>MTIDINKLKEELGLGDLAKSLEGLTAAQKAQEAERMRKEQEEKELARMNDLVSKAVGEDRKRLEEALELVKSLDEKSKKSNELFAQTVEKQQETIVGLQDEIKSLLTAREGRSFVGDSVAKALYGTQENFEDEVEKLVLLSYVMEKGVFETEHGQRHLKAVNQSSSVEVSSESYETIFSQRIIRDLQKELVVGALFEELPMSSKILTMLVEPDAGKATWVAASTYGTDTTTGEEVKGALKEIHFSTYKLAAKSFITDETEEDAIFSLLPLLRKRLIEAHAVSIEEAFMTGDGSGKPKGLLTLASEDSAKVVTEAKADGSVLVTAKTISKLRRKLGRHGLKLSKLVLIVSMDAYYDLLEDEEWQDVAQVGNDSVKLQGQVGRIYGLPVVVSEYFPAKANSAEFAVIVYKDNFVMPRQRAVTVERERQAGKQRDAYYVTQRVNLQRYFANGVVSGTYAAS[12x];>[2x]MIDYSGLRTIFGEKLPESHIFFATVAAHKYVP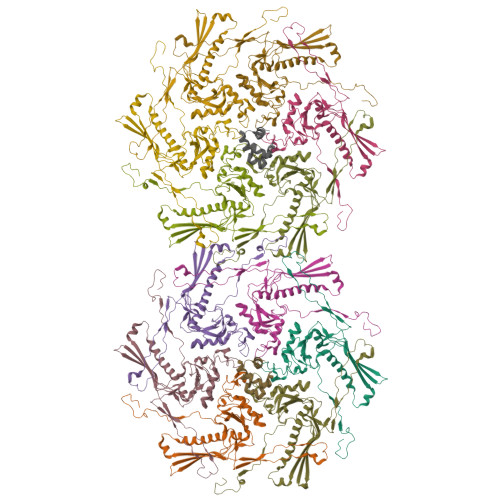SYAFLRRELGLSSAHTNRKVWKKFVEAYGKAIPPAPPAPPLTLSKDLTASMSVEEGAALTLSVTATGGTGPYTYAWTKDGSPIPDASGATYTKPTAAAEDAGSYKVTVTDSKQVSKDSTTCAVTVNPTVPGG Thymidine kinase (TK) catalyses the transfer of the γ-phosphate of ATP to 2’-deoxythymidine (dThd) forming thymidine monophosphate (dTMP). L. major Type II TK (LmTK) has been previously shown to be important for infectivity of the parasite and therefore has potential as a drug target for anti-leishmanial therapy. The enzymes from Leishmania spp. are type II TKs with a ~100 amino acid C-terminal extension compared to those from other species. The overall structure of the LmTK catalytic domain in all three complexes shows a nearly identical fold to those of type II TKs from other species, as expected from the sequence identity of ~50% on the amino acid level.

The end product of the thymidine salvage pathway, dTTP, exerts strong feedback inhibition, limiting the phosphorylation of lethal nucleoside analogues or DNA chain terminators both in mam006Dalian and in T. brucei TKs. The determination of the IC50 value for dTTP was performed at increasing dTTP concentrations using saturating concentrations of ATP (0.5 mM) and dThd (25 μM) and gave a value of 3.8 ± 0.07 μM and a positive Hill coefficient (h = 1.6). The LmTK–dTTP crystal has a well-resolved dTTP in the thymidine-binding site, the magnesium being coordinated by the phosphates, in all eight protomers in the asymmetric unit. The residues around the dTTP have essentially the same conformation as in the dThd complex, with the exception of E85 that is turned away from the 5’-oxygen of the ribose ring, no longer forming a hydrogen bond. In most chains of the LmTK structures this loop is also disordered. While in LmTK-dTTP it can be traced in two out of the eight chains, this is an artefact of crystallization as it forms an additional β-strand to the central β-sheet of a symmetry-related tetramer in the crystal lattice. The LmTK-dThd and LmTK-AP5dT crystals contain two protomers per asymmetric unit, with the tetramer sitting on a crystallographic 2-fold axis, while the LmTK-dTTP asymmetric unit contains two tetramers. LmTK forms closed tetramers in all three complexes, which explains the lack of density for the adenine in LmTK-dThd and its unexpected position in LmTK-AP5dT.

>MSGHHHHHHFRGRIELIIGPMFAGKTTELMRRVKREIHARRSCFVIKYSKDTRYDEHNVASHDQLMLRAQAAVSQLTEVRDTWKRFDVLAIDEGQFFSDLVDFCNTAADAGKVVMVSALDGDYRRKPFGQICELVPYCEAVDKLTAVCMMCHEQPACFTRRTVNVEQQELIGGADMYIATCRECYSKQQLP[8x]The PH domain-containing protein Slm1 from budding yeast Saccharomyces cerevisiae is required for actin cytoskeleton polarization and cell growth. The PH domain-containing protein Slm1 from S. cerevisiae is a component of the target of rapamycin complex 2 (TORC2) signaling pathway. We have previously reported that in vitro, the Slm1-PH domain (Slm1-PH) interacts with liposomes containing PtdIns(4,5)P2 and DHS-1P cooperatively. The core of each monomer consists of seven antiparallel β-strands with a C-terminal amphipathic α-helix connected via a long and flexible loop.

The results presented here include: (i) the apo structure of Slm1-PH that we resolved at 1.76 Å resolution; (ii) one structure with phosphoserine at 1.68 Å resolution; and (iii) two structures of Slm1-PH in complex with Ins(4)P at 1.4 and 1.8 Å resolution. Electron densities corresponding to the Ins(4)P molecules were visible between the β1-β2 and β5-β6 loop regions (difference density maps). For the two structures determined in complex with Ins(4)P, the positions of the inositol ring overlap. In both cases, the oxygen atoms of the inositol ring contact the β1-β2 region through the hydroxyl group of Tyr485 (hydrogen bond length  = 2.8 Å) and the NH2 group of Arg478 (hydrogen bond length  = 2.5 Å), and the β5-β6 loop through the ε-amino group of Lys542 (hydrogen bond length  = 2.7 Å). In addition, we observed a contact with the ε-amino group of Lys562 (hydrogen bond length  = 3.2 Å) from the β6-β7 strand. Interestingly, the two structures differ with respect to the orientation of the phosphate at position 4 (P4), which contacts either the β1-β2 loop or turns 180° and contacts the β5-β6 loop. In the first case, the main-chain nitrogen of Tyr485 and the carbonyl oxygen of Ser484 (hydrogen bond lengths  = 3.0 and 3.1 Å, respectively) of the β1-β2 loop region interact with P4, whereas in the other structure the main-chain nitrogen atom of Ser539 of the β5-β6 loop forms hydrogen bonds of 2.6 Å with the oxygen atom of P4. Also in Slm1-PH, the most conserved positively charged residue within the β1-β2 loop (Arg478) is flipped towards the non-canonical binding site to interact with the Ins(4)P molecule. The non-canonical binding site is shallow, large and solvent-exposed, and so the phosphate position of Ins(4)P in one of the structures was seen on the opposite side of the molecule. * Crystals of the same protein-ligand complex were obtained in different crystallization conditions.

>DHPFTEIKSGFLERRSKFLKSYSKGYYVLTPNFLHEFKTADRKKDLVPVMSLALSECTVTEHSRKNSTSSPNSTGSDAKFVLHAKQNGIIRRGHNWVFKADSYESMMSWFDNLKILTSTS[4x]>GAMGSDEEQSPDWDSHGLPANIVVQLNKLSGFKKYKVSDIMFFDRRRQTTIGTEDSFFEMVSIRPGGVYTKAQLQKELETLATCGMFEKVDLEGKTKPDGTLGVTISFAESTWQSADRFRCINVGLMVQSKPIEMDSDMTDKEKLEYYRSLEKDYKRRIDRARPCLLPAPVYGEVMQMLRDQGKVSARLLQRIRDRVQKWYHDEGYACAQVVNFGNLNTKEVVCEVVEGDITQLVIQFQDKLGNVVEGNTQVPVVRRELPKQLRQGYVFNIEAGKKALSNINSLGLFSNIEVNPRPDEKNEGGI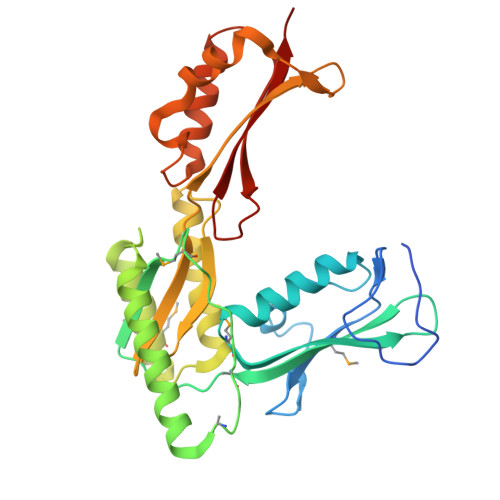IVEIKLKELE[2x]> AAPANAVTADDPTAIALKYNQDATKSERVAAARPGLPPEEQHCANCQFMQANVGEGDWKGCQLFPGKL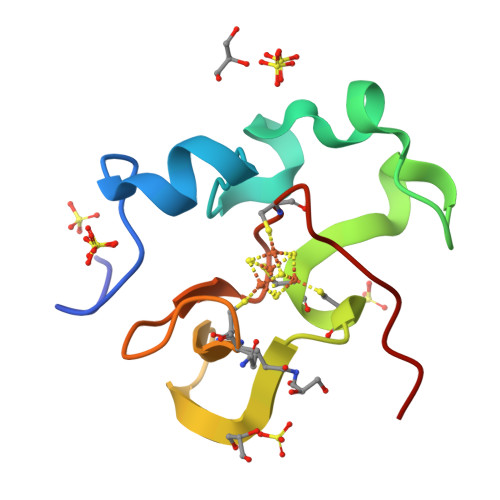INVNGWCASWTLKAG> SQGHKPLEVIKIEDGVYLHTSFKNIEGYGLVDSNGLVVLDNNQAYIIDTPWSEEDTKLLLSWATDRGYQVMASISTHSHEDRTAGIKLLNSKSIPTYTSELTKKLLAREGKPVPTHYFKDDEFTLGNGLIELYYPGAGHTEDNIVAWLPKSKILFGGCLVRSHEWEALGYVGDASISSWADSIKNIVSKKYPIQMVVPGHGKVGSSDILDHTIDLAESASNK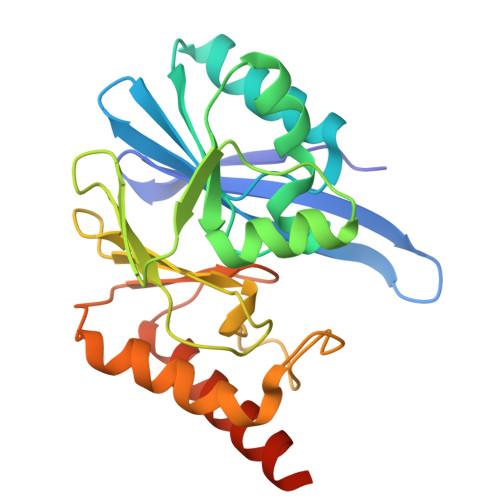LMQPTAEASAD N-(naphthalen-2-yl)methanimine | C11 H9 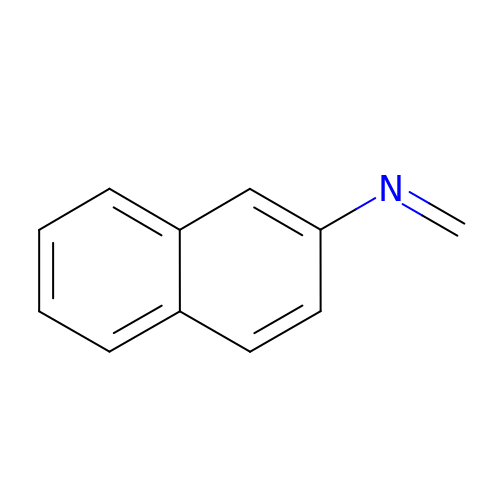N | FGRABSHVUNBHIE-UHFFFAOYSA-N> ANPLYQKHIISINDLSRDDLNLVLATAAKLKANPQPELLKHKVIASCFFEASTRTRLSFETSMHRLGASVVGFSDSANTSLGKKGETLADTISVISTYVDAIVMRHPQEGAARLATEFSGNVPVLNAADASNQHPTQTLLDLFTIQETQGRLDNLHVAMVGDLKYGRTVHSLTQALAKFDGNRFYFIAPDALAMPQYILDMLDEKGIAWSLHSSIEEVMAEVDILYMTRVQKERLDPSE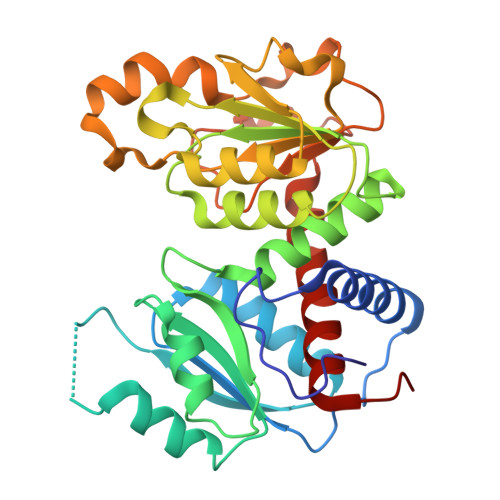YANVKAQFVLRASDLHNAKANMKVLHPLPRVDEIATDVDKTPHAWYFQQAGNGIFARQALLALVLNRDLVL>MKRAVITGLGIVSSIGNNQQEVLASLREGRSGITFSQELKDSGMRSHVWGNVKLDTTGLIDRKVVRFMSDASIYAFLSMEQAIADAGLSPEAYQNNPRVGLIAGSGGGSPRFQVFGADAMRGPRGLKAVGPYVVTKAMASGVSACLATPFKIHGVNYSISSACATSAHCIGNAVEQIQLGKQDIVFAGGGEELCWEMACEFDAMGALSTKYNDTPEKASRTYDAHRDGFVIAGGGGMVVVEELEHALARGAHIYAEIVGYGATSDGADMVAPSGEGAVRCMKMAMHGVDTPIDYLNSHGTSTPVGDVKELAAIREVFGDKSPAISATRAMTGHSLGAAGVQEAIYSLLMLEHGFIAPSINIEELDEQAAGLNIVTETTDRELTTVMSNSFGFGGTNATLVMRKLKD[4x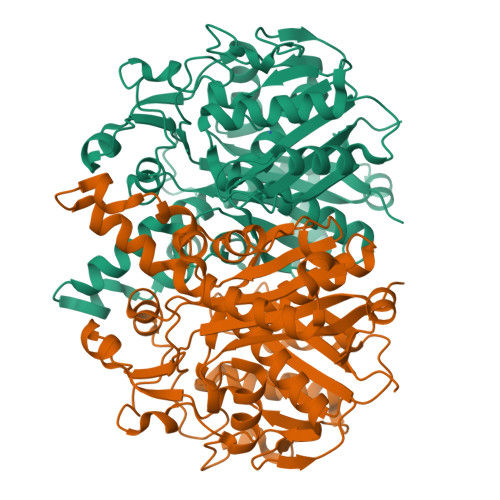]> FGLLFVGFVAGGVAGGYFWGRSNGGGGGASVSSTQAGFDKIGKDIQQLRNDTNAAIEGFNGRIAHDEQAIKNL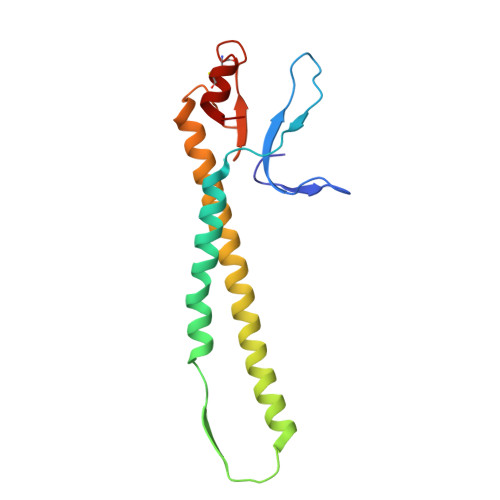AKEIEDARAEALVGELGIIRSLIVANISMNLKESLYELANQITKRGGGIAQEAGPGCWYVDSENCDASCKEYIFNF CYTIDINE-5'-MONOPHOSPHATE-5-N-ACETYLNEURAMINIC 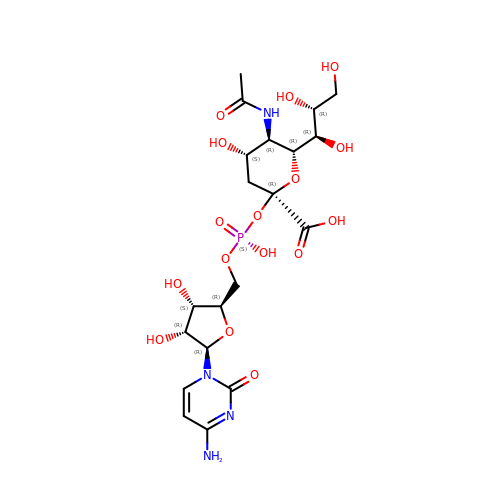ACID | C20 H31 N4 O16 P | TXCIAUNLDRJGJZ-BILDWYJOSA-N>MHKDVKAIYEESKILDEATHLYGVQRSDIHFIADAENYVYELKKDGESFILKITHTIRRSPDYILGEMEWLHHLAKGGLSVAKPIASLNGRDIEQVDDGQGGSFLLRVYEKAPGHKVEEADWNDELFYALG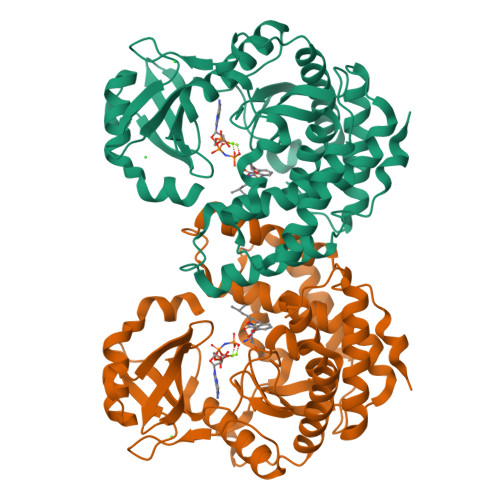QYTGRMHKLTKSYQLSDPRYKRQEWDEEEQLKLRKYVPADQTLVFEQADRLMEKLAKLPKNQDTYGLVHADLHHGNFHWDQGKITTFDFDDIGYNWFMNDISILLYNVLWYPVIPYEDKAAFAGNFMKQFLKGYREENELGDEWLAYIPDFLRLRHVLIYGLLHQAFDLATIGDEEKAMLASFRSDIEQAAPITTFDFTKLSQS[4x]>[2x]AKEMKPFPQQVNYAGVIKPNHVTQESLNASV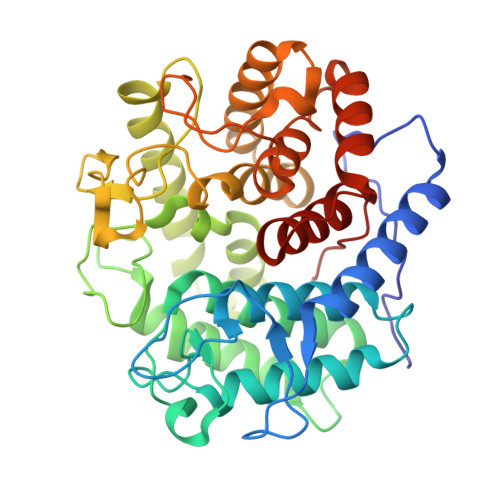RSYYDNWKKKYLKNDLSSLPGGYYVKGEITGDADGFKPLGTSEGQGYGMIITVLMAGYDSNAQKIYDGLFKTARTFKSSQNPNLMGWVVADSKKAQGHFDSATDGDLDIAYSLLLAHKQWGSNGTVNYLKEAQDMITKGIKASNVTNNNQLNLGDWDSKSSLDTRPSDWMMSHLRAFYEFTGDKTWLTVINNLYDVYTQFSNKYSPNTGLISDFVVKNPPQPAPKDFLDESEYTNAYYYNASRVPLRIVMDYAMYGEKRSKVISDKVSSWIQNKTNGNPSKIVDGYQLNGSNIGSYPTAVFVSPFIAASITSSNNQKWVNSGWDWMKNKRERYFSDSYNLLTMLFITGNWWKPVP>[4x]VPLLLSGHTEAALREQSTRLLNDLLEHPDEHPADVGYTLITGRAHFGHRAAVIGESREELLDALKALAEGREHHTVVRGDGTAHPDRRVVFVFPGQGSQWPSMARDLLDRAPAFRETAKACDAALSVHLDWSVLDVLQEKPDAPPLSRVDVVQPVLFTMMLSLAACWRDLGVHPAAVVGHSQGEIAAACVAGALSLEDAARIV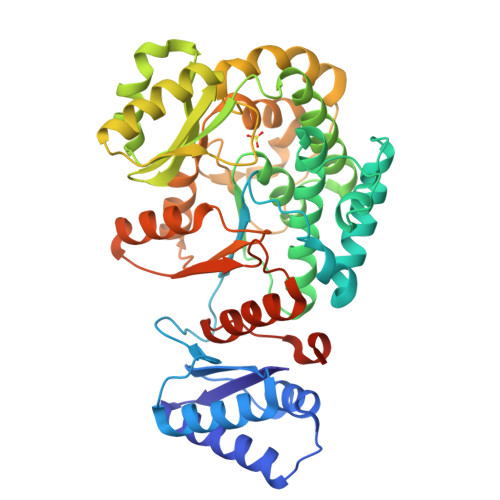ALRSRAWLTLAGKGGMAAVSLPEARLRERIERFGQRLSVAAVNSPGTAAVAGDVDALRELLAELTAEGIRAKPIPGVDTAGHSAQVDGLKEHLFEVLAPVSPRSSDIPFYSTVTGAPLDTERLDAGYWYRNMREPVEFEKAVRALIADGYDLFLECNPHPMLAMSLDETLTDSGGHGTVMHTLRRQKGSAKDFGMALCLAYVNGLEIDGEALFGPDSRRVNPPTYPFQ>[5x]STLHISDLILQASPVVQLVMLILLLASIFSWYLIAKLHMSYKKARQDDEHFQKMFWSGAELNTLYNNAQLNSKRSGLEDIFYQGLSEFFKLKKRQAPTSQMIEGTERILRVGLSRDQGSLEYGLGTLASIGSVAPYIGLFGTVWGIMNAFIGLAAVDQVTLATVAPGIAEALI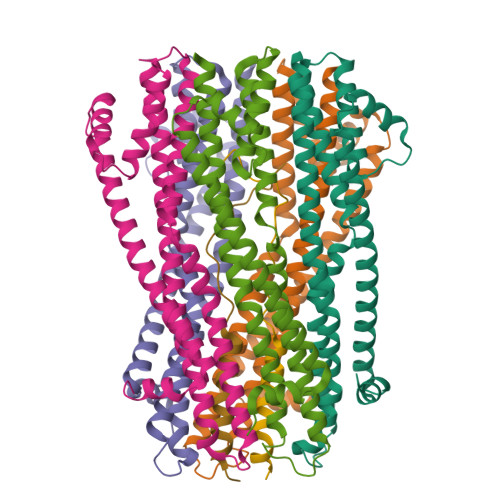ATAIGLFAAIPAVLAFNHFTAKSESVYSDRALFAEEMIALLQRQSVG;>[2x]GRFERIKKPLKSDMNVVPYIDVMLVLLVIFMVTAPMITS> MTSASEPSGPSGSAPVLIVGGSLVGLSTAVFLARHGVRCTLVERHPGTSVHPRAVGYYPRTGELLRQAGVEDAAVREASGFATHRTRAGVTSLAGEVLFSKEELEGDDDLGDLTPSRLLLLPQDRLEPLLRDRAVELGADLRFGTELVSFAEDPEGVTAVLDDGTGGTRTFRSSYLVACDGPRS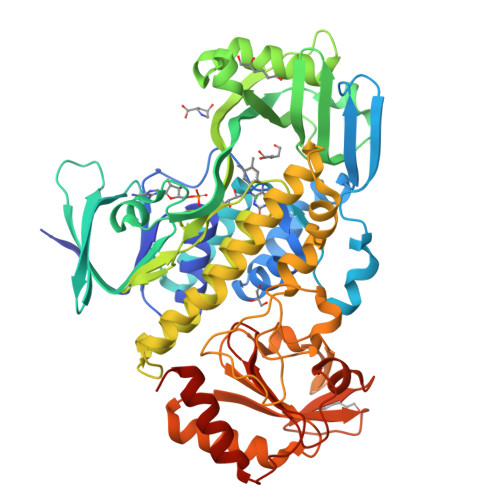TVREALKVPRQGRGVLSRHVSIAFGADLRPVLGDRRYSVVHVKNPQVTGILVHDDTLTGGTLIVGYRPEDGESLEDFTDDRCAELVGAAVGAPGVEVTIRSRFPWDMAEQVAESFVHGRVLLAGDAAHVVPPTGGYGANTGIADAHNLAWKLALVAAGVAGPGLVETYDAERRPVAVYTAEQGSLQLALRSGTATPEQQAAVADAVTVTSGQAYRSTAVVGEPDGADLPVASDPRELRGAPGTRAPYVELLRGGETVSTLDLFGRDFVLLTGEHGREWISAAVSASAGLGLKITARRVVPGTDAGAGTLADPDGDWSERYGGLRPEGAVLVRPDGVVAWRSPGADPGGEESAVLAAVLRSVLARESRTGGK>[8x]MSTDRTGNIVGKMIAAINAVIKDEKVSYSEYKASTGWLISVGEKNEWPLFLDVFFEHAIESVAAESNRGSQSSIQGPYFIPGAPELSIPYTMPMRDDESGDTLIFRGEVVDQEGAPLAD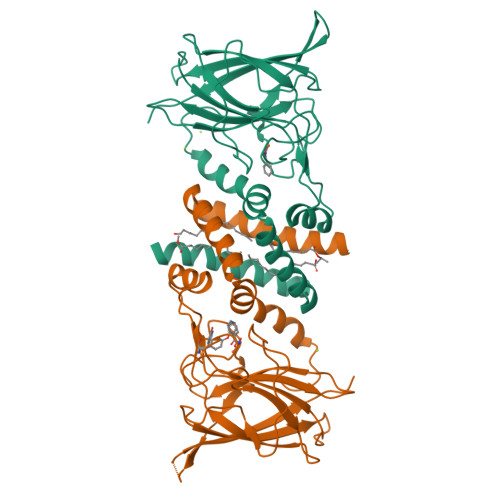VLLDMWQADAAGEYSFINPTLPDYLFRGKIRTDENGRFTLRTIVPAPYEIPKNGPTGALLAAAGWHAWRPAHLHWIIAKEGYESLTTQLYFENGQWTGSDVANAVKPELLLSLDKIEAQSGPHFETSYKFTLGKV>DESQVPDQPSSLHVRPQTNCIIMSWTPPLNPNIVVRGYIIGYGVGSPYAETVRVDSKQRYYSIERLESSSHYVISLKAFNNAGEGVPLYESATTRGSGGSGGSGGSGGSGGSGGSG[2x];>[2x]GMLPPVGVQAVALTHDAVRVSWADNSVPKNQKTSEVRLYTVRWRTSFSASAKYKSEDTTSLSYTATGLKPNTMYEFSVMVTKNRRSSTWSMTAHATTYEAAPTSAPKDLTVITREGKPRAVIVSWQPPLEANGKITAYILFYTLDKNIPIDDWIMETISGDRLTHQIMDLNLDTMYYFRIQARNSKGVGPLSDPILFRTLKLEVLFQ

Deleted in colorectal cancer (DCC) is a single pass transmembrane glycoprotein that was originally identified in humans as a candidate tumor suppressor. DCC belongs to the immunoglobulin superfamily, and the extracellular fragment is composed of four immunoglobulin-like (Ig-like) domains followed by six fibronectin type III (FN) domains. DCC plays a pivotal role in axon guidance by mediating a combination of attractive and repulsive effects through interactions with the diffusible guidance cue, netrin-1 and draxin. Located between the functional DCCFN4 and DCCFN5 domains is an 8–28 amino acid linker, which is contingent on the particular DCC isoform.

Here we have undertaken a structural and functional analysis of the DCC construct DCCFN456, with a 22-residue long “artificial” linker composed of Ser-Gly-Gly (SGG) repeats (herein referred to as SGG-22) between the FN4 and FN5 domains. The DCC construct that was expressed in E. coli and crystallized contained a linker of 22 amino acids, and the linker is represented as G(SGG)7. Since there is a 22-residue linker between the FN4 and FN5 domains, which is disordered in the crystal structure and can potentially stretch somewhere around 80 Å, we cannot authenticate which FN4 domain is linked to which FN5 domain to form one molecule. In the concave-shaped CFG β sheet, a group of hydrophobic residues M921, W931, Y895 and the aliphatic portion of side chains from R884 and R865 emanated from different strands stack on top of one another, forming a “hydrophobic ladder”. The critical residues involved in the netrin-1 binding to site 1 and site 2 cluster on either side of this hydrophobic ladder, respectively. A stable, solid FN5 domain has therefore evolved to serve a key role in netrin-1 binding, able to resist the force generated by the binding from the either side. In the crystal lattice of the structure we determined, four FN4 domains are positioned around one rod-like FN5-FN6 entity. We then would like to propose that this configuration of FN4-A-linker-FN5-FN6 molecule might represent a stable “resting” state of the DCC receptor.>MRVLGIETSCDATGIAIYDDEKGLLANQLYSQVKLHADYGGVVPELASRDHVRKTVPLIQAALKESGLTAKDIDAVAYTAGPGLVGALLVGATVGRSLAFAWDVPAIPVHHMEGHLLAPMLEDNPPEFPFVALLVSGGHTQLISVTGIGQYELLGESIDDAAGEAFDKTAKLLGLDYPGGPLLSKMAAQGTAGRFVFPRPMTDRPGLDFSFSGLKTFAANTIRDNGTDDQTRADIARAFEDAVVDTLMIKCKRALDQTGFKRLVMAGGVSANRTLRAKLAEMMKKRRGEVFYARPEFCTDNGAMIAYAGMVRFKAGATADLGVSVRPRWPLAELPAAHHHHHH[2x];>MRILAIDTATEACSVALWNDGTVNAHFELCPREHTQRILPMVQDILTTSGTSLTDINALAYGRGPGSFTGVRIGIGIAQGLALGAELPMIGVSTLMTMAQGAWRKNGATRVLAAIDARMGEVYWAEYQRDENGIWHGEETEAVLKPEIVHERMQQLSGEWVTVGTGWQAWPDLGKESGLVLRDGEVLLPAAEDMLPIACQMFAEGKTVAVEHAEPVYLRNNVAWKKLPGKEHHHHHH[2x]

The N6-threonylcarbamoyladenosine (t6A) modification at position 37 of ANN-decoding tRNAs is one of the few modifications that are found in the three domains of life. In the first half of the reaction, YrdC utilizes ATP, L-threonine and bicarbonate to synthesize an unstable intermediate TCA, whose threonylcarbamoyl-moiety is subsequently transferred onto the adenosine at position 37 of the substrate tRNAs by the cooperative action of three proteins YeaZ, YgjD and YjeE. In archaea and yeast, the transfer reaction requires the kinase, putative endopeptidase and other proteins of small size (KEOPS) protein complex, composed of Kae1, Bud32, Cgi121 and Pcc1, complemented by a fifth fungi-specific protein Gon7 in yeast. It is now well established that YgjD and its orthologs Kae1 and Qri7 are responsible for the catalysis of the transfer reaction. YgjD and YeaZ are forming a heterodimer that is capable of interacting with YjeE.

We wanted to analyze the importance of the Mg2+ ion, by mutating its Glu12 carboxylate ligand into alanine. The crystal structure of YgjDE12A–YeaZ in complex with ATP determined at 2.3 Å confirmed the absence Mg2+ in the active site. Interestingly, this mutant has ATP bound at the active site compared to ADP for the wild YgjD–YeaZ type although no binding of AMPCPP to YgjDE12A was observed by ITC. YgjD probably has a very weak ATPase activity, which is inhibited in the YgjDE12A mutant, explaining why we observed ATP at the active site of the mutant. Moreover, there was no electron density observed for ADP at the YgjDE12A–YeaZ interface, suggesting this site could have a preference for ADP rather than ATP. We observed that the in vitro t6A activity of YgjDE12A is totally abolished. However the ATPase activity of the ternary complex YgjDE12A–YeaZ–YjeE is not affected by this mutation. These data further confirm that YgjD is responsible for the t6A coupling reaction and YgjE for ATP hydrolysis.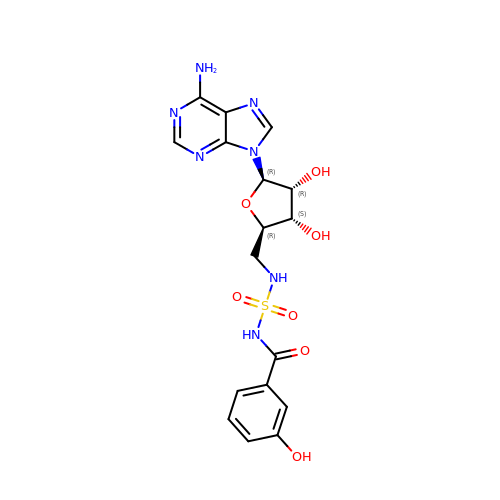5'-deoxy-5'-{[(3-hydroxybenzene-1-carbonyl)sulfamoyl]amino}adenosine | C17 H19 N7 O7 S | DNCWBHYPLQFCLB-CNEMSGBDSA-N>GNSDDARTSIEQRSNAVSQVLLGIFSYVRWPKEPAVLQLCVVGPTEYA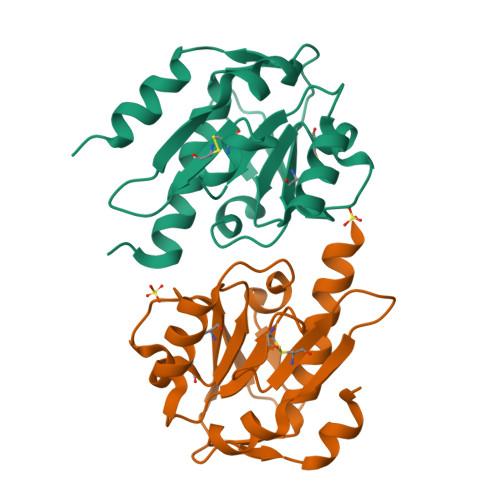DGLLRGMVQANGRRVHAERRAVDNPDLGTLCNVIYLGVVDERERQQVFRSLAGHPVLSISERGTECSVGSMFCLNVGGPRITFEANLDSIARSGVRVHPSVLKLARRQATP[4x]> Q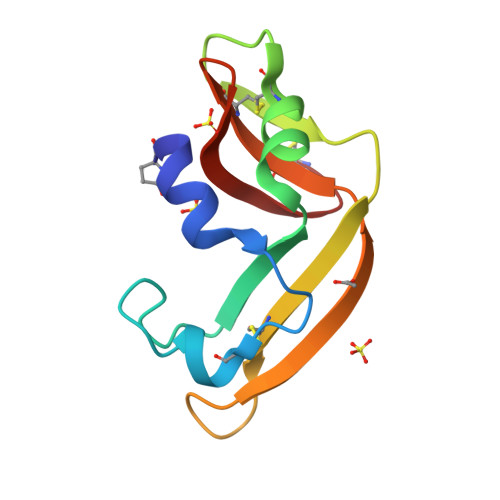DWLTFQKKHITNTRDVDCDNIMSTNLFHAKDKNTFIYSRPEPVKAICKGIIASKNVLTTSEFYLSDCNVTSRPAKYKLKKSTNKFCVTCENQAPVHFVGVGSC>[4x]EAEASNMSSAH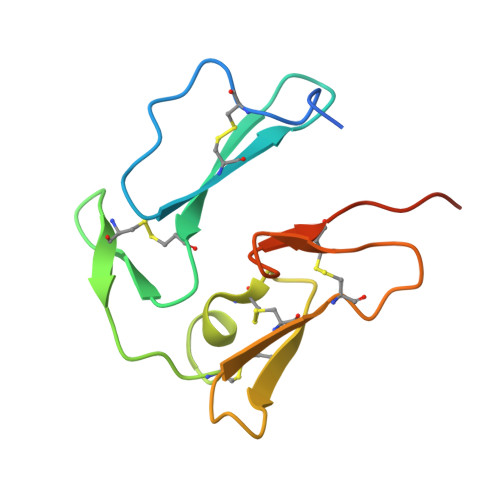KCIDTNVPENAACYRYLDGTEEWRCLLGFKEVGGKCVPASITCEENNGGCAPEAECTMDDKKEVECKCTKEGSEPLFEGVFCSSSSGPHHHHHH> SASPA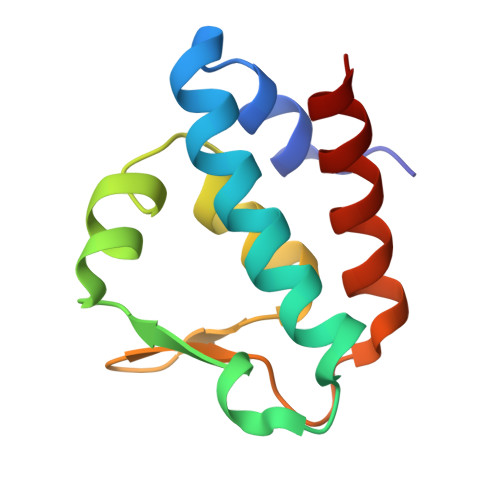VAELCQNTPETFLEASKLLLTYADNILRNPSDEKYRSIRIGNTAFSTRLLPVRGAVECLFEMGFEEGETHLIFPKKASVEQLQKIRDLIAIERSS>MAASLPSTLSFSSAPDEIQHPQIKFSEWKFKLFRVRSFEKAPEEAQKEKDSSEGKPYLEQSPVVPEKPGGQNSILTQRALKLHPKFSKKFHADGKSSDKAVHQARLRHFCRICGNRFKSDGHSRRYPVHGPVDAKTQSLFRKKEKRVTSWPDLIARIFRIDVKADVDSIHPTEFCHDCWSIMHRKFSSSHSQVYFPRKVTVEWHPHTPSCDICFTAHRGLKRKRHQPNVQLSKKLKTVLNHARRDRRKRTQARVSSKEVLKKISNCSKIHLSTKLLAVDFPAHFVKSISCQICEHILADPVETSCKHLFCRICILRCLKVMGSYCPSCRYPCFPTDLESPVKSFLNILNSLMVKCPAQDCNEEVSLEKYNHHVSSHKESKETLVHINKGGRPRQHLLSLTRRAQKHRLRELKIQVKEFADKEEGGDVKAVCLTLFLLALRARNEHRQADELEAIMQGRGSGLQPAVCLAIRVNTFLSCSQYHKMYRTVKAITGRQIFQPLHALRNAEKVLLPGYHPFEWQPPLKNVSSRTDVGIIDGLSGLASSVDEYPVDTIAKRFRYDSALVSALMDMEEDILEGMRSQDLDDYLNGPFTVVVKESCDGMGDVSEKHGSGPAVPEKAVRFSFTVMRITIEHGSQNVKVFEEPKPNSELCCKPLCLMLADESDHETLTAILSPLIAEREAMKSSELTLEMGGIPRTFKFIFRGTGYDEKLVREVEGLEASGSVYICTLCDTTRLEASQNLVFHSITRSHAENLQRYEVWRSNPYHESVEELRDRVKGVSAKPFIETVPSIDALHCDIGNAAEFYKIFQLEIGEVYKHPNASKEERKRWQATLDKHLRKRMNLKPIMRMNGNFARKLMTQETVDAVCELIPSEERHEALRELMDLYLKMKPVWRSSCPAKECPESLCQYSFNSQRFAELLSTKFKYRYEGKITNYFHKTLAHVPEIIERDGSIGAWASEGNQSGNKLFRRFRKMNARQSKCYEMEDVLKHHWLYTSKYLQKFMNAHNALKSSGFTMNSKETLGDPLGIEDSLESQDSMEF[2x];>MSLQMVTVGHNIALIQPGFSLMNFDGQVFFFGQKGWPKRSCPTGVFHFDIKQNHLKLKPAIFSKDSCYLPPLRYPATCSYKGSIDSDKHQYIIHGGKTPNNELSDKIYIMSVACKNNKKVTFRCTEKDLVGDVPEPRYGHSIDVVYSRGKSMGVLFGGRSYMPSTQRTTEKWNSVADCLPHVFLIDFEFGCATSYILPELQDGLSFHVSIARNDTVYILGGHSLASNIRPANLYRIRVDLPLGTPAVNCTVLPGGISVSSAILTQTNNDEFVIVGGYQLENQKRMVCSLVSLGDNTIEISEMETPDWTSDIKHSKIWFGSNMGNGTIFLGIPGDNKQAMSEAFYFYTLRCSEEDLSEDQKIVSNSQTSTEDPGDSTPFEDSEEFCFSA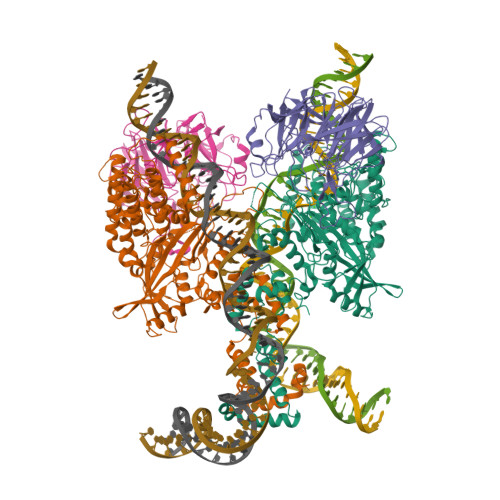EATSFDGDDEFDTYNEDDEDDESVTGYWITCCPTCDVDINTWVPFYSTELNKPAMIYCSHGDGHWVHAQCMDLEERTLIHLSEGSNKYYCNEHVQIARALQTPKRNPPLQKPPMKSLHKKGSGKVLTPAKKSFLRRLFD[2x]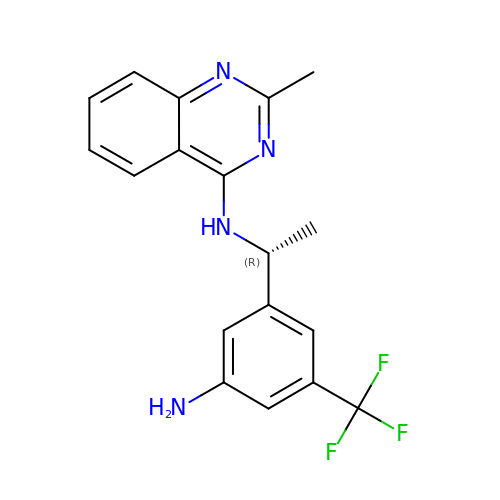~{N}-[(1~{R})-1-[3-azanyl-5-(trifluoromethyl)phenyl]ethyl]-2-methyl-quinazolin-4-amine | C18 H17 F3 N4 | CVDHTLSRRHNJAW-SNVBAGLBSA-N> MKVLPKLALANLVCFTTLSVFAQPADPSGQQTSTNTSNLVTYLTNLGKYLGYDITQSSKAPNPPYSQLFNSNVVQLVQNYAYNTFLGAIPVDAMSQSLMNFVTDKVQGNSLINNLANTTFKYQNFSAPSSGADGKITANGLIDQSTASAQTPTTPGIFSAPQITTSGTYLNDPVSQAVFNILGTPDYSFCMDNEQKNWLPNCNLMYQNLVMQNVIGTLPPAQTSGSTPAFYSYKYNQPLISQLNSNSLIAPLLMDTSASQSGQDSGLTAKSQAQQALNFIRYASAQVTPPSLPKLSAYSELWNQATAKPN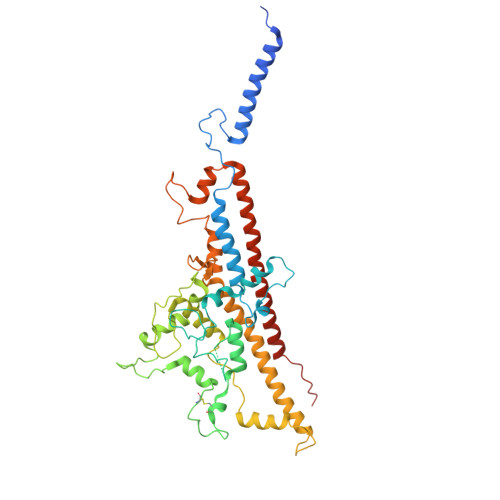SAGYNEVQQKQAAATLSSYFNNLRVYAAQTSVGVSNLYYILSKRLPQNMSADQSNANITSQALNEFNMATRRLFDPTASNTPGQPNQQWIKQINDASPATVQKEIAILLAEINYQMYLDRQIQERILLTNSIMLLQNLKAAQPTADFSSQGSPSEQ2'-deoxy-5-[(4-ethynylphenyl)ethynyl]cytidine 5'-(tetrahydrogen triphosphate) | C19 H20 N3 O13 P3 | 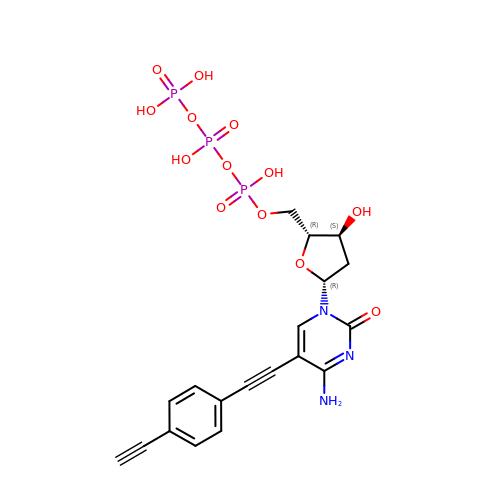CPJFKEBWOPVPDF-GVDBMIGSSA-N>[2x]MTKPDFTGARERFLAGDVTIVLLIAESHDAPYRLANPEDPEADLSDEQLERALAAYLTLVETLFPELYAEMKAALAAAKTPEEKIAVFREYN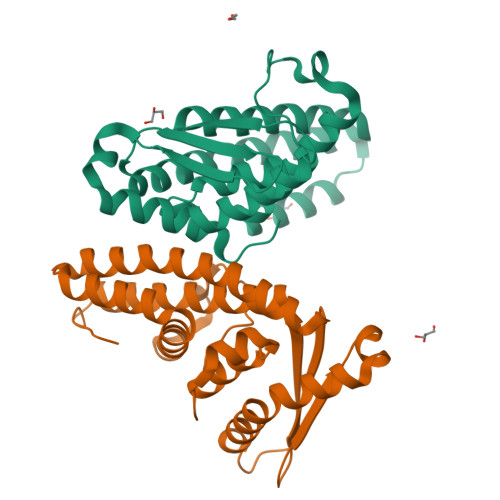ARFLAEFDALIDQAFARLKADSLTLKIHLSQGKGSYEIIFPPEVQADPERAAAIEALWKPTLDQLLAVLQEKHKGKPATTVTYEISAETLRAAVAALARAAEAALRRKVGSLESSGLEVLFQ>STVYSAKGTSLEVGGRAEARLSLKDGKAQDNSRVRLNFLGKAEINDSLYGVGFYEGEFTTNDQGKNASNNSLDNRYTYAGIGGTYGEVTYGKNDGALGVITDFTDIMSYHGNTAAEKIAVADRVDNMLAYKGQFGDLGVKA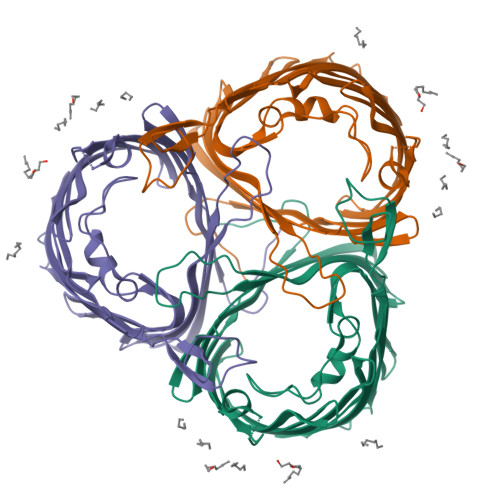SYRFADRNAVDAMGNVVTETNAAKYSDNGEDGYSLSAIYTFGDTGFNVGAGYADQDDQNEYMLAASYRMENLYFAGLFTDGELAKDVDYTGYELAAGYKLGQAAFTATYNNAETAKKTSADNFAIDATYYFKPNFRSYISYQFNLLDSDKASKVASEDELAIGLRYDF[2x]>GSHMTATTGPPPKLCLVCSDEASGCHYGV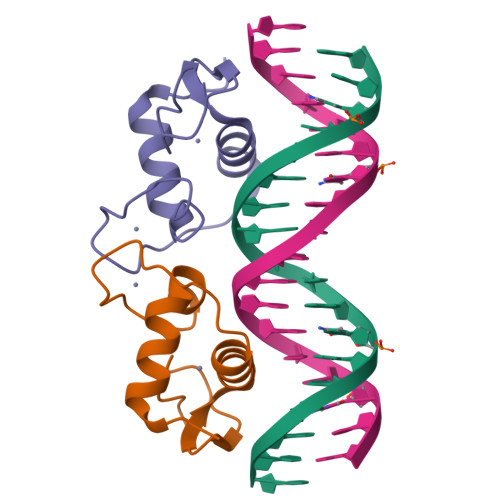LTCGSCKVFFKRAVEGQHNYLCAGRNDCIIDKIRRKNCPACRYRKCLQAGMNLEARKTKKKIKGI[2x]>[2x]MEFKDFPLKPEILEALHGRGLTTPTPIQAAALPLALEGKDLIGQARTGTGKTLAFALPIAERLAPSQERGRKPRALVLTPTRELALQVASELTAVAPHLKVVAVYGGTGYGKQKEALLRGADAVVATPGRALDYLRQGVLDLSRVEVAVLDEADEMLSMGFEEEVEALLSATPPSRQTLLFSATLPSWAKRLAERYMKNPVLINVIKDEPVTYEEEAVPAPVRGRL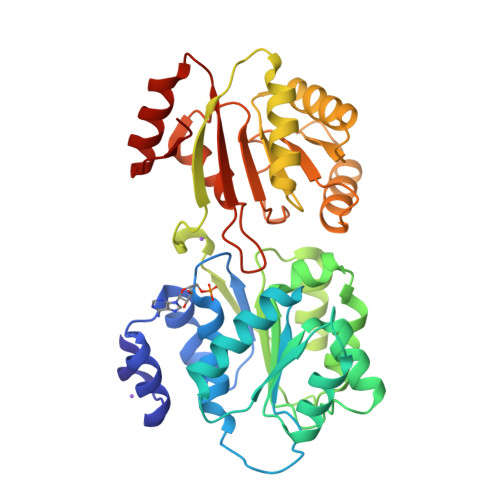EVLSDLLYVASPDRAMVFTRTKAETEEIAQGLLRLGHPAQALHGDLSQGERERVLGAFRQGEVRVLVATDVAARGLDIPQVDLVVHYRLPDRAEAYQHRSGRTGRAGRGGRVVLLYGPRERRDVEALERAVGRRFKRVN Sulfur, essential to many biomolecules such as sulfur-containing amino acids and cofactors including iron-sulfur cluster, is usually mobilized from cysteine by the pyridoxal 5′-phosphate- (PLP-) dependent enzyme of cysteine desulfurase (CDS). We determined the crystal structures of CDS from Thermococcus onnurineus NA1 (ToCDS), which include native internal aldimine (NAT), gem-diamine (GD) with alanine, internal aldimine structure with existing alanine (IAA), and internal aldimine with persulfide-bound Cys356 (PSF) structures. ToCDS belongs to class II CDS based on the primary and tertiary structures and showed the highest similarity with EcSufS. ToCDS is a PLP-dependent enzyme and the crystallographic snapshots of catalytic intermediates of ToCDS showed the conserved dihedral angle rotation of Schiff-base linkage relative to the PLP pyridine ring as shown in EcNifS_CsdB and XometC, which implies the PLP-dependent catalytic mechanism of ToCDS is well conserved.

The crystal structure of native ToCDS (NAT) was determined to be 2.6 Å. There was a dimer with a twofold symmetry in the asymmetric unit. A protomer of ToCDS comprised three domains. The larger central domain having PLP binding site contained residues 17–285 and comprised nine α-helices surrounding a nine β-stranded, mainly parallel β-sheet. The two active sites were located in the center of the PLP-binding domain at the dimer interface. PLP was Schiff-base linked with Lys216 at the active site. The PLP pyridine ring was well stacked with His114 and bound to Ala192 with van der Waals interaction at the opposite side. 5′-phosphate of PLP was tightly bound via hydrogen bonds with the nearby residues of Ser87, His215, Ser213, and Thr268. However, the internal dihedral angle showed flexible conformational changes from 38° to 69°: the internal dihedral angle got wider in the order of NAT, IAA, and GD structures.

>MHHHHHHSSENLYFQGHMASMRIPEDVRKDIPLTNEVIYFDNTATSLTPKPVVEAMDEYYLKYRANVHRGVHRLSQMATHKYEESRKIVADFIGAKFEEIVFTKNTSESLNLVALGLGHIFKRGDKIVTTPYEHHSDLLPWQRLATKLGLKLEFIEGDDEGNLDLSDAEKKIKGAKLVAVQHVSNALGVIHEVEELGKIAKDEGAIFVVDAAQSAGHMEVNVKKLHADFLAFSGHKGPMGPTGIGVLYIREEFFDTFEPPLIGGGTIEDVSLDGYKLTEPPERFEAGTPNIGGAIGLAAGIRYIERIGLGRIERQEHKLVKRTTEGLDELEVPWYGPRNLKKHAGVVSFNVPGLHPHDVAAILDDHSIMVRSGHHCALPVMKKLGINGTVRASFHVYNSLEEVETFLGVMEELVKGLKT[2x]6-amino-2-(methylamino)-3,7-dihydro-8H-imidazo[4,5-g]quinazolin-8-one | C10 H10 N6 O | 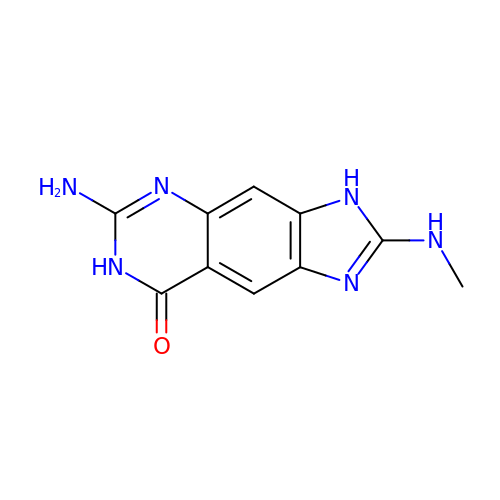MRAWGMPHZYODAJ-UHFFFAOYSA-N> DYKLFITEGYEVGRVNGLAVIGESAGIVLPIIAEVTPSMSKSEGRVIATGRLQEIAREAVMNVSAIIKKYTGRDISNMDVHIQFVGTYEGVAGDSASISIATAVISAIEGIPVDQSVAMTGSLSVKGEVLPVGGVTQ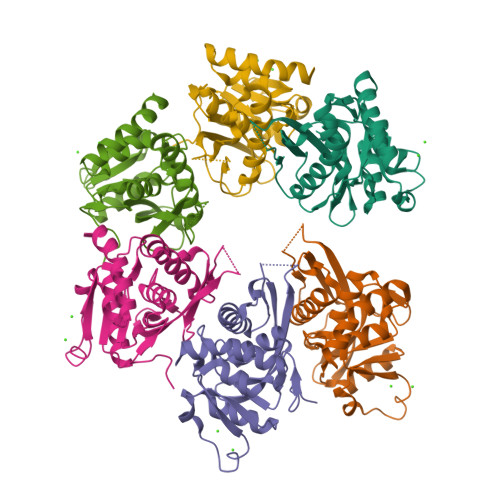KIEAAIQAGLKKVIIPKDNIDDVLLDAEHEGKIEVIPVSRINEVLEHVLEDGKKKNRLMSKFKELELAAV2-[(2~{E},6~{E},10~{Z},14~{E},18~{E},22~{E},26~{E})-3,7,11,15,19,23,27,31-octamethyldotriaconta-2,6,10,14,18,22,26,30-octaenyl]naphthalene-1,4-dione 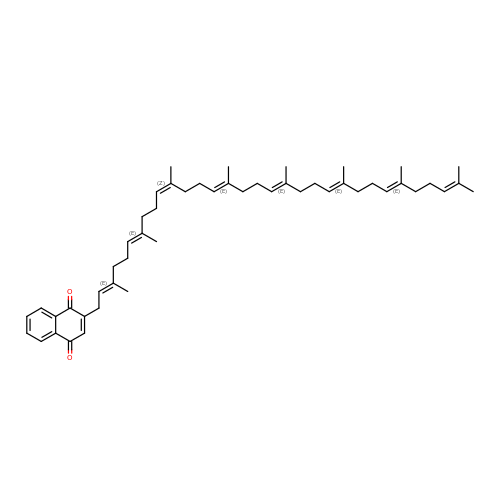| C50 H70 O2 | GDUBPWSFXUAETN-FTDSSYSJSA-N>MTYSVSPSSLLTEYGNDNICRVLALDGGGAKGFYTLGVLKEIEAMLGCPLYKRFDLVFGTSTGAIIAALIALGYEVDQIHALYTEHVPRVMSSRSAAARTMALQDLAKEVFQDKTFEDVLMGIGIVATRWMTERPMIFKGNVVQAHGRKGTFSPGFGVSIADAVQASCSAYPFFERKVIVTAAGDKVELIDGGYCANNPTLFAIADATVALKKDHKDIRVINVGVGIYPEPKPGLLMRIAKKWLAVQLLQKTLEIN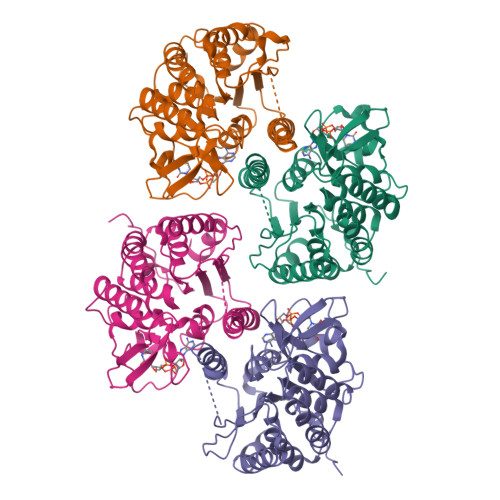TQSMDQLRDILFKDIPTIRISDTFERPEMATDLLEYNLDKLNTLRQRGRESFGAREAQLREFLI[4x]>[6x]MKNKVVVVTGVPGVGGTTLTQKTIEKLKEEGIEYKM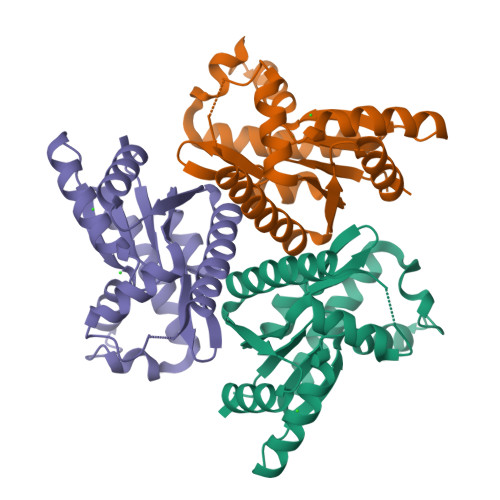VNFGTVMFEVAKEEGLVEDRDQMRKLDPDTQKRIQKLAGRKIAEMAKESNVIVDTHSTVKTPKGYLAGLPIWVLEELNPDIIVIVETSSDEILMRRLGDATRNRDIELTSDIDEHQFMNRCAAMAYGVLTGATVKIIKNRDGLLDKAVEELISVLKLEHHHHHH> R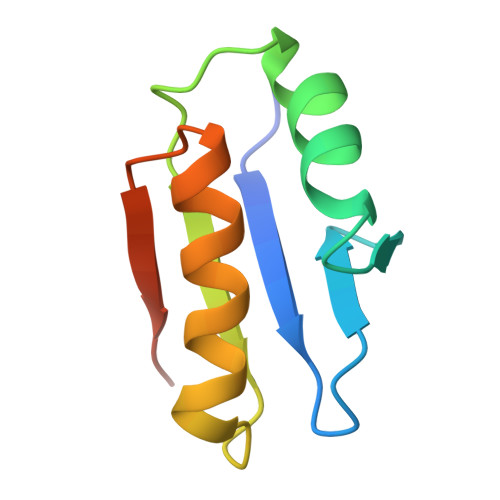PEKPVYLSVKADNSMFIGNDPVTDETMITALNALTEGKKDTTIFFRADKTVDYETLMKVMDTLHQAGYLKIGLVGEETAKAK>[8x]MAHHHHHHMNASSDLQATLDPSRKSWVESANNPTGDFSIQNLPFGIFSDGLNATRRVGVAIGDSIVDLAALESAGLLSVPSTGAGDSVFVRDALNDFIALGRDAWRSVRVQLSRLLSRDDATLRDDA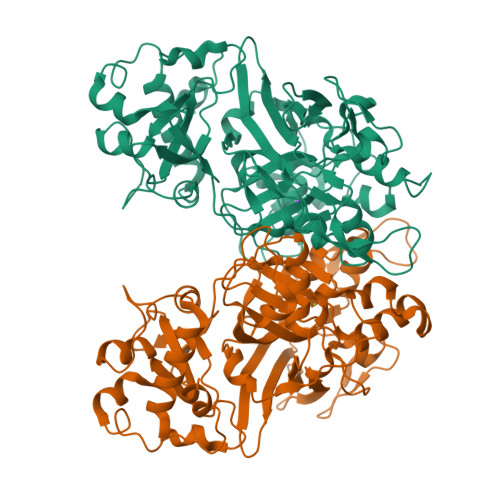ELRGRALIRQADAQLHLPVQIPGYTDFYSSKEHATNVGSMFRDPKNALLPNWSEMPIGYNGRASSVVVSGTPVRRPNGQLKLPDQERPVFGACRKLDIELETGFVIGAGNALGEPVTCADAEAHIFGMVLLNDWSARDIQQWEYVPLGPFNAKTFATTISPWIVTLDALEPFRVAQPAQDPQPLAYLRHDGEHAFDITLEVTLRPQQAKEASTITRTNFKHMYWTMAQQLAHHTVSGCNTRVGDLMGSGTISGPTEDSFGSLLELTWNGKKPLELREGGTRSFIEDGDELTLAGWCQGEGYRVGFGVCAGEILPALK>[6x]MA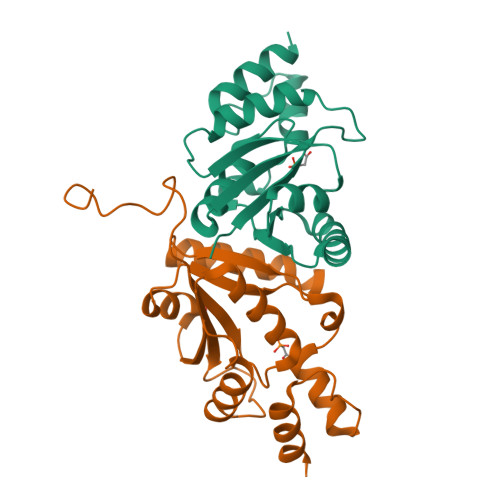SMTGGQQMGRGSMSTKAIYPGTFDPITNGHIDIITRAASMFDRVILAIAASPSKKPMFDLEERVALATTALQHLPNVEVMGFSDLMANFARAQQANILIRGLRAVADFEYEMQLAHMNRHLMPELESVFLMPSKEWSFISSSLVKEVARHAGDVTHFLPANVHQALMEKLK> MDLCQIPPTSPISPSVPFNGDDSSVVRRSANYPANLWDYDFLQSLGRHSSVTEEHVGLAEKLKGEVKSLITGPMEPLAKLEFIDSVRRLGLKYQFETEMKEALANISKDGYDSWWVDNLRATALRFRLLRENGIFVPQDVFERFQNKETGKFKNELCEDV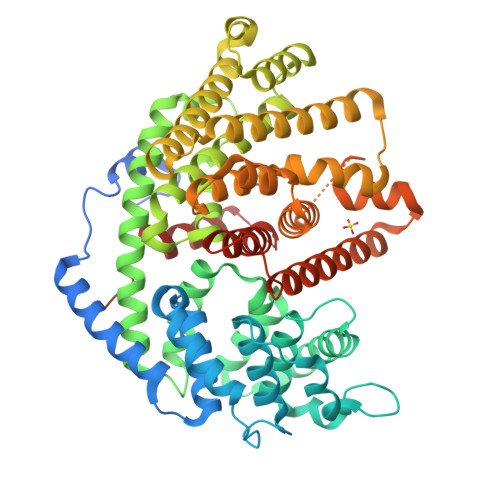KGLLNLYEASFLGWEGEDILDEARTFSTAQLKNVEGKISSPNLAKIVHHALDLPLHWRAIRYEARWFIDIYEDEEDMNPTLLKYAKLDFNIVQSFHQAEIGRLARWWVGTGLDKLPFARNGLIQSYMYAIGMLFEPHLGEVREMEAKVGALITTIDDVYDVYGTMEELELFTDITERWDINRVDQLPRNIRMPLLTMFNTSNDIGYWALKERGFNGIPYTAKVWADQLKSYTKEAKWFHEGHKPTLEEYLENALVSIGFPNLLVTSYLLTVDNPTKEKLDYVDSLPLFVRASCILCRIINDLGTSPDEMERGDNLKSIQCYMNETGASQEVAREHIEGLVRMWWKRLNKCLFEPSPFTEPFLSFTINVVRGSHFFYQYGDGYGNAESWTKNQGMSVLIHPITLDEE> MEQNLFALSLDDTSSVRGSLLDTKFAQTRVLLSKAMAGGDVLLDEYLYDVVNGQDFRATVAFLRTHVITGKIKVTATTNISDNSGCCLMLAINSGVRGKYSTDVYTICSQDSMTWNPGCKKNFSFTFN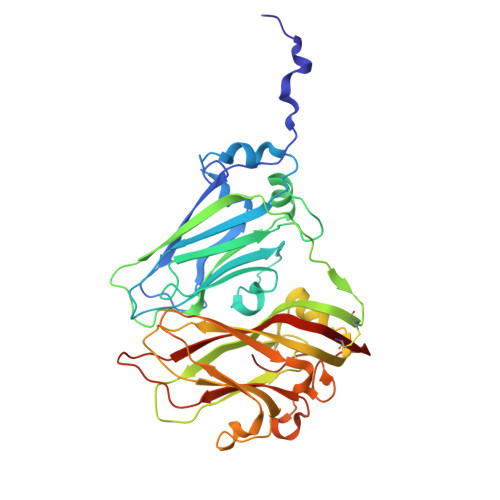PNPCGDSWSAEMISRSRVRMTVICVSGWTLSPTTDVIAKLDWSIVNEKCEPTIYHLADCQNWLPLNRWMGKLTFPQGVTSEVRRMPLSIGGGAGATQAFLANMPNSWISMWRYFRGELHFEVTKMSSPYIKATVTFLIAFGNLSDAFGFYESFPHRIVQFAEVEEKCTLVFSQQEFVTAWSTQVNPRTTLEADGCPYLYAIIHDSTTGTISGDFNLGVKLVGIKDFCGIGSNPGIDGSRLL> PIVRVAVLAAGDDGGRLTEMALPSELPLREILPAVQRIVQPARENDGAADPAAAPNPVRLSLAP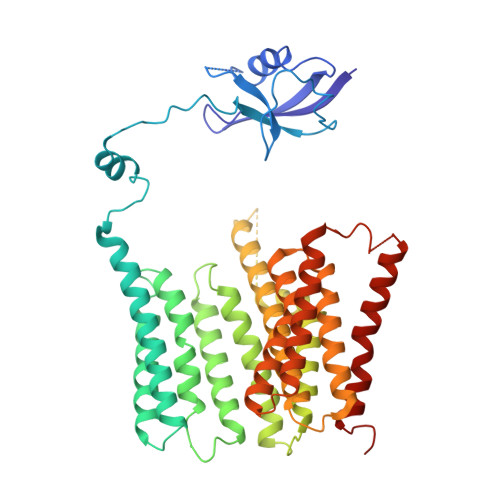IGGAPFSLDATLDTVGVVDGDLLALQAVPSGPPAPRIVEDIADAAVIFSEARRRQWGPTHIARGAALALIGLILVGTGLSVAHRVITGDLLGQFIVSGIALATVIAALAVRNRSAVLATSLAVTALVPVAAAFALGVPGDFGAPNVLLAAAGVAAWSLISMAGSPDDRGIAVFTATAVTGVGVLLVAGAASLWVISSDVIGCALVLLGLIVTVQAAQLSAMWARFPLPVIPAPGDPTPAARPLSVLADLPRRVRVSQAHQTGVIAAGVLLGVAGSVALVSSANASPWAWYIVVAAAAGAALRARVWDSAACKAWLLGHSYLLAVALLVAFVIGDRYQAALWALAALAVLVLVWIVAALNPKIASPDTYSLPMRRMVGFLATGLDASLIPVMALLVGLFSLV> SNANDPPNIPNVTGPT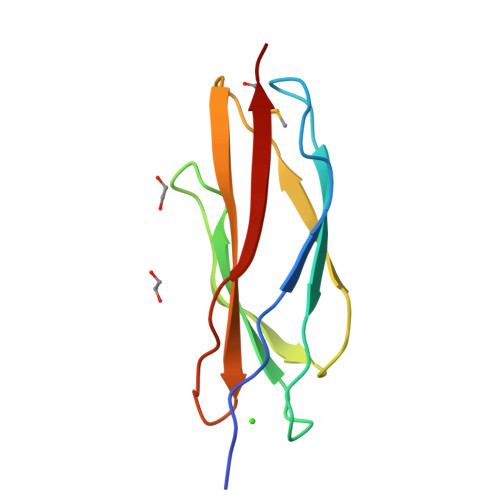NGNIGTTYNYTFVTTDPNGDNITYYIEWGDGFTEEWIGPYASGEEVIFSHTWDKKGTYVVRAKAKDILNYESSWGTLEVTMPK> GHMNLYRSRNFYARIRGDRALFTNPATKGGSERSSYSVPTRQALQGIIDGIYHKPTFTNVITEVKVVNQIQTELHGVRALLHDYSADLSYVSYLSDVEYLVKFHFIWNENREDLIQDRLPKKHEAIMERSIRKGG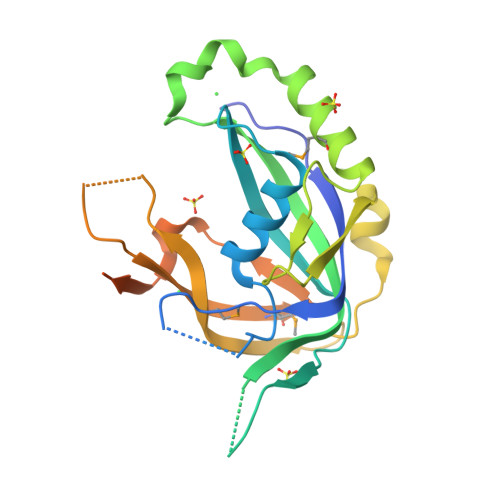RRDIFLGTRECFGLVDEISQEEYETIPSYYNGVTIDLGIMFHSFAYPTSKDTPLKSYFTKTVMENGAIKFKPQSECEIVNTLSSYAFKSLGQLKSVDDEYVDDEYEEYEAMEKGEGGS> MSLKYIIGMDVGTTATKGVLYDINGKAVASVSKGYPLIQTKVGQAEEDPKLIFDAVQEIIFDLTQKIDGKIAAISWSSQMHSLIGLGSDDELLTNSITWADNCAKSIVQDAKNRGFAQQIYRKTGMPMHPMAPIYKLLWLKNKKTEVFSQAQKWIGIKEYIIFRLTGKLVTDTTMAAGTGILNLKTLTWDQELLDILKIKKEQLPKIAQPTKVIFPIKTEYVKKLGIDSDTKIILGASDGYLSTIGVNAIDSDHCALNVGTSGAIRTIVDQPKIDPSASYFCYPADKTHYLLGGPVNNGGIVFNWARQTLFDADETPQDFLDVAQTAPAGSRNLIFLPYLGGERAPIWDANARGSFVGLTRMHQKPEMARAVIEGIIFNLYDAASNL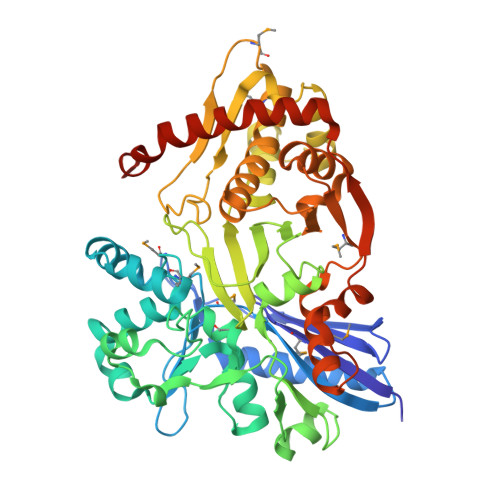IKNTKKPVAINATGGFLKSDFVRQLCANIFNVPIVTMKEQQSGTLAAMFLARQALGLNQDLSEIGQFAQADKVYFPNPKEAATYQKLFPLYCEIRNALAASYGKFSNINEGHHHHHH4-{4-[2-(2,3-dihydro-1H-indol-1-yl)-2-oxoethyl]phenyl}phthalazin-1(2H)-one | C24 H19 N3 O2 | 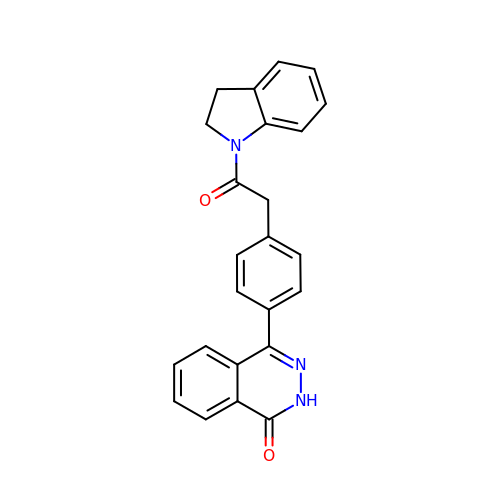COYVFENBIAJDFY-UHFFFAOYSA-N5-deoxy-5-fluoro-D-xylulose | C5 H9 F O4 | 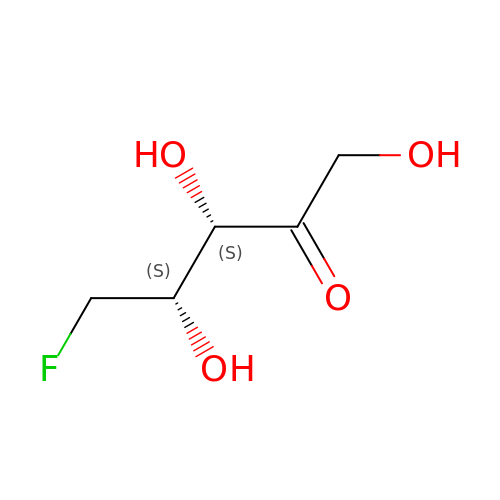DZPAPJMTQBXJAM-WUJLRWPWSA-N> PPPAIGQFWHVTDLHLDPTYHITDDHTKVCASSKGANASNPGPFGDVLCDSPYQLILSAFDFIKNSGQEASFMIWTGDSPPHVPVPELSTDTVINVITNMTTTIQSLFPNLQVFPALGNHDYWPQDQLPVVTS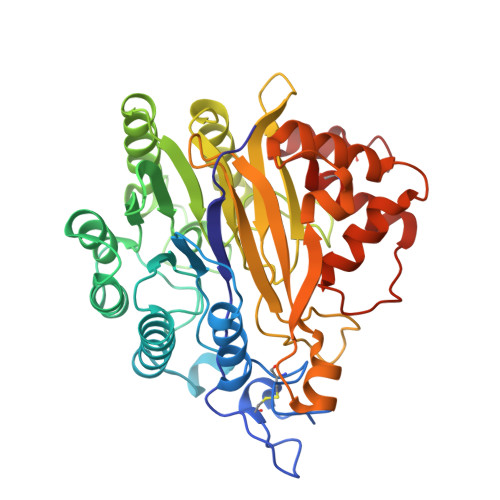KVYNAVANLWKPWLDEEAISTLRKGGFYSQKVTTNPNLRIISLNTNLYYGPNIMTLNKTDPANQFEWLESTLNNSQQNKEKVYIIAHVPVGYLPSSQNITAMREYYNEKLIDIFQKYSDVIAGQFYGHTHRDSIMVLSDKKGSPVNSLFVAPAVTPVKSVLEKQTNNPGIRLFQYDPRDYKLLDMLQYYLNLTEANLKGESIWKLEYILTQTYDIEDLQPESLYGLAKQFTILDSKQFIKYYNYFFVSYDSSVTCDKTCKAFQICAIMNLDNISYADCLKQL>[3x]MIFEKAVIVDLRTQVLDVPV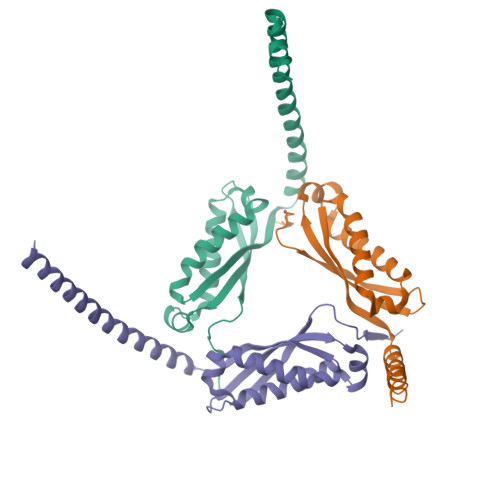QETITKDNVPVRVNAVVYFRVVDPVKAVTQVKNYIMATSQISQTTLRSVIGQAHLDELLSERDKLNMQLQRIIDEATDPWGIKVTAVEIKDVELPAGMQKAMARQAEAERERRARITLAEAERQAAEKLREAAEIISEHPMALQLRTLQTISDVAGDKSNLEHHHHHH> SHMEK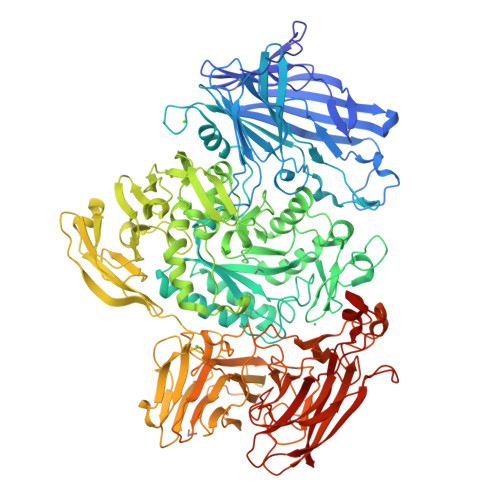ETGPEVDDSKVTYDTIQSKVLKAVIDQAFPRVKEYSLNGHTLPGQVQQFNQVFINNHRITPEVTYKKINETTAEYLMKLRDDAHLINAEMTVRLQVVDNQLHFDVTKIVNHNQVTPGQKIDDESKLLSSISFLGNALVSVSSDQTGAKFDGATMSNNTHVSGDDHIDVTNPMKDLAKGYMYGFVSTDKLAAGVWSNSQNSYGGGSNDWTRLTAYKETVGNANYVGIHSSEWQWEKAYKGIVFPEYTKELPSAKVVITEDANADKNVDWQDGAIAYRSIMNNPQGWEKVKDITAYRIAMNFGSQAQNPFLMTLDGIKKINLHTDGLGQGVLLKGYGSEGHDSGHLNYADIGKRIGGVEDFKTLIEKAKKYGAHLGIHVNASETYPESKYFNEKILRKNPDGSYSYGWNWLDQGINIDAAYDLAHGRLARWEDLKKKLGDGLDFIYVDVWGNGQSGDNGAWATHVLAKEINKQGWRFAIEWGHGGEYDSTFHHWAADLTYGGYTNKGINSAITRFIRNHQKDAWVGDYRSYGGAANYPLLGGYSMKDFEGWQGRSDYNGYVTNLFAHDVMTKYFQHFTVSKWENGTPVTMTDNGSTYKWTPEMRVELVDADNNKVVVTRKSNDVNSPQYRERTVTLNGRVIQDGSAYLTPWNWDANGKKLSTDKEKMYYFNTQAGATTWTLPSDWAKSKVYLYKLTDQGKTEEQELTVKDGKITLDLLANQPYVLYRSKQTNPEMSWSEGMHIYDQGFNSGTLKHWTISGDASKAEIVKSQGANDMLRIQGNKEKVSLTQKLTGLKPNTKYAVYVGVDNRSNAKASITVNTGEKEVTTYTNKSLALNYVKAYAHNTRRNNATVDDTSYFQNMYAFFTTGADVSNVTLTLSREAGDEATYFDEIRTFENNSSMYGDKHDTGKGTFKQDFENVAQGIFPFVVGGVEGVEDNRTHLSEKHDPYTQRGWNGKKVDDVIEGNWSLKTNGLVSRRNLVYQTIPQNFRFEAGKTYRVTFEYEAGSDNTYAFVVGKGEFQSGRRGTQASNLEMHELPNTWTDSKKAKKATFLVTGAETGDTWVGIYSTGNASNTRGDSGGNANFRGYNDFMMDNLQIEEITLTGKML2-phenylmethoxyaniline | C13 H13 N O | 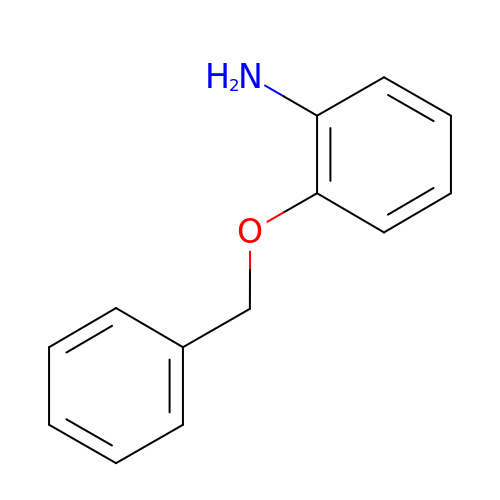PLPVLSBYYOWFKM-UHFFFAOYSA-N>[4x]MGSDKIHHHHHHMVIGQKVL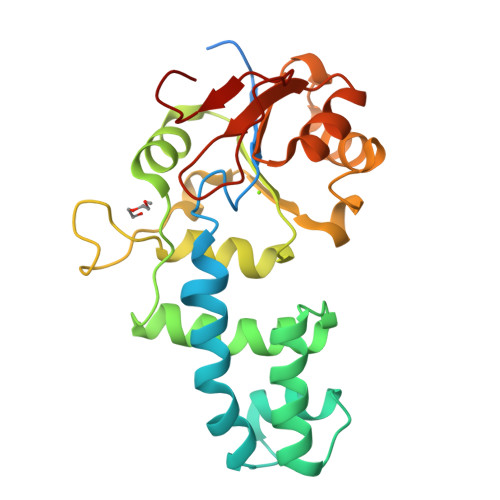LARIPKMGDNYSTYLLDIEGTVCPISFVKETLFPYFTNKVPQLVQQDTRDSPVSNILSQFHIDNKEQLQAHILELVAKDVKDPILKQLQGYVWAHGYESGQIKAPVYADAIDFIKRKKRVFIYSSGSVKAQKLLFGYVQDPNAPAHDSLDLNSYIDGYFDINTSGKKTETQSYANILRDIGAKASEVLFLSDNPLELDAAAGVGIATGLASRPGNAPVPDGQKYQVYKNFETL> MSQNLFNVEDYRKLAQKRLPKMVYDYLEGGAEDEYGVKHNRDVFQQWRFKPKRLVDVSRRSLQAEVLGKRQSMPLLIGPTALNGALWPKGDLALARAATKAGIPFVLSTASNMSIEDLARQCDGDLWFQLYVIHREIAQGMVLKALHTGYTTLVLTTDVAVNGYRERDLHNRFKIPPFLTLKNFEGIDLGKMDKANLEMQAALMSRQMDASFNWEALRWLRDLWPHKLLVKGLLSAEDADRCIAEGADGVILSNHGGRQLDCAISPMEVLAQSVAKTGKPVLIDSGFRRGSDIVKALALGAEAVLL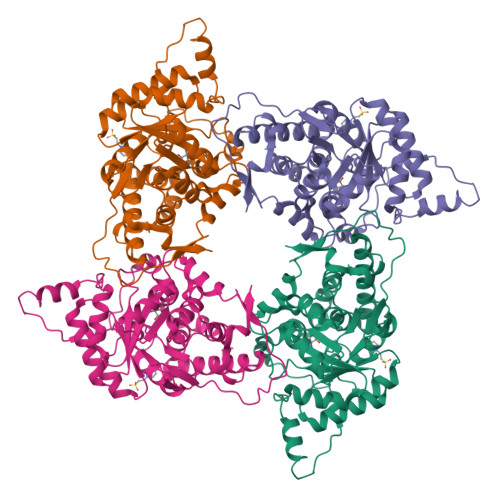GRATLYGLAARGETGVDEVLTLLKADIDRTLAQIGCPDITSLSPDYLQNEGVTNTAPVDHLIGKGTHAHHHHHH> SNASADAQSFLNRVCGVSAARLTPCGTGTSTDVVYRAFDIYNDKVAGFAKFLKTNCCRFQEKDEDDNLIDSYFVVKRHTFSNYQHEETIYNLLKDCPAVAKHDFFKFRIDGDMVPHISRQRLTKYTMADLVYALRHFDEGNCDTLKEILVTYNCCDDDYFNKKDWYDFVENPDILRVYANLGERVRQALLKTVQFCDAMRNAGIVGVLTLDNQDLNGNWYDFGDFIQTTPGSGVPVVDSYYSLLMPILTLTRALTAESHVDTDLTKPYIKWDLLKYDFTEERLKLFDRYFKYWDQTYHPNCVNCLDDRCILHCANFNVLFSTVFPPTSFGPLVRKIFVDGVPFVVSTGYHFRELGVVHNQDVNLHSSRLSFKELLVYAADPAMHAASGNLLLDKRTTCFSVAALTNNVAFQTVKPGNFNKDFYDFAVSKGFFKEGSSVELKHFFFAQDGNAAISDYDYYRYNLPTMCDIRQLLFVVEVVDKYFDCYDGGCINANQVIVN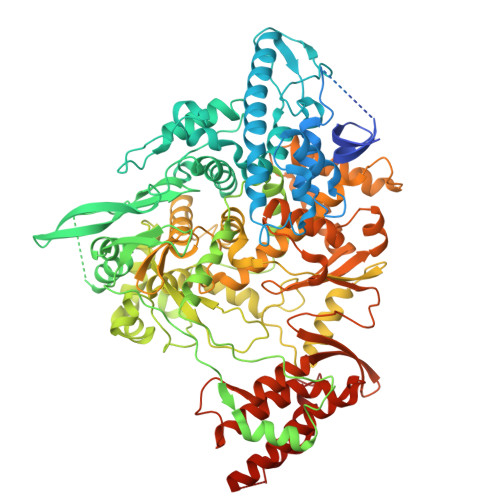NLDKSAGFPFNKWGKARLYYDSMSYEDQDALFAYTKRNVIPTITQMNLKYAISAKNRARTVAGVSICSTMTNRQFHQKLLKSIAATRGATVVIGTSKFYGGWHNMLKTVYSDVENPHLMGWDYPKCDRAMPNMLRIMASLVLARKHTTCCSLSHRFYRLANECAQVLSEMVMCGGSLYVKPGGTSSGDATTAYANSVFNICQAVTANVNALLSTDGNKIADKYVRNLQHRLYECLYRNRDVDTDFVNEFYAYLRKHFSMMILSDDAVVCFNSTYASQGLVASIKNFKSVLYYQNNVFMSEAKCWTETDLTKGPHEFCSQHTMLVKQGDDYVYLPYPDPSRILGAGCFVDDIVKTDGTLMIERFVSLAIDAYPLTKHPNQEYADVFHLYLQYIRKLHDELTGHMLDMYSVMLTNDNTSRYWEPEFYEAMYTPHTVLQ1-methylsulfonylethane 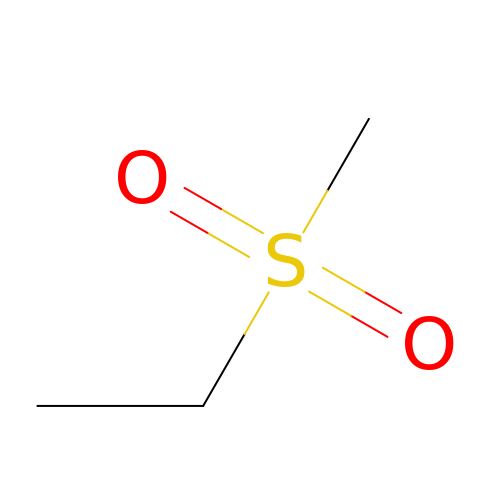| C3 H8 O2 S | YBJCDTIWNDBNTM-UHFFFAOYSA-N N-{(3S,4S)-4-[(6-aminopyridin-2-yl)methyl]pyrrolidin-3-yl}ethane-1,2-diamine 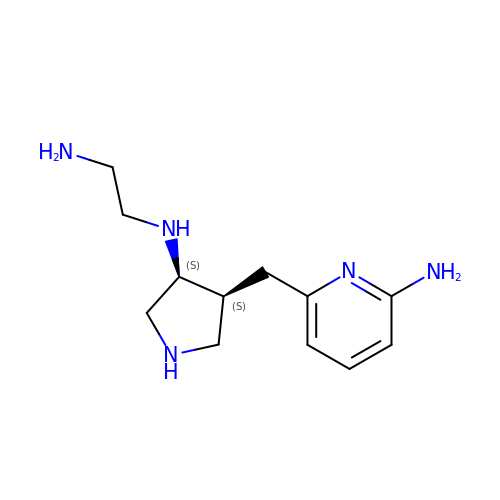| C12 H21 N5 | BETYXZSFUFTOLC-GXSJLCMTSA-N> MWILESELFDGKRLWLRPGKTYLFGRTVAEAGQLTISDKTVSRKHLTIHIDNVPEGGGRNLRSRSNVIVEDLESKKGTLVNGVQIRGQKTTLTEDVNEIKLGLCPKTLKIRWHPIVLSFSFTSKELRADPWTNLRDSLEQLDIKYSAEYEPTTTHVVSKKRNTSKGLQALINGRYIVTDSFINAIVQATEIPEGEEGASSALEQDFEANWPNPLDHLPPRGEEPGNHTTETYAPDARRQEVFDGYTFIFYEKKQYDNLFPAISAGKGKALLKEVVPNRTRVDEFVRYVKSVAGEKGLGSFEDGSEGKGVVVVRYTPKGEDSAWYAEFFTKFAQQLDHRPIDQKEFLEAILACDASMLRRPLEAMSQPVSVSASVEPQSSEKVRPAVEDRKEVEQ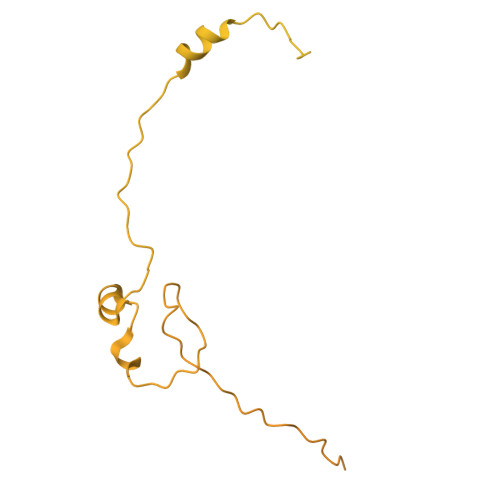SAPKQLQPSAEVPATEESAPAPHRRERRTGRSRFKGFDFDDDDIIIETPQAQSSTQVPALPQVPSASQDSLFVSQREPSLAPSEPMLEEEAPCNTRTTRQTHRKRVLSPLPEHDNSALLDEIAPITAAVKRRRIEAGQDPVPPLPEPEPEREDEDVEMVEESPPRKGKKGAATTAKGKGKKIKQEDEENVLELARRRREEAEAAAAAERQRLAQLGDDDIDYAAIRRLHIIEEIEVRQPEPHGPNRTREQDIADGRWDPRWNGRKNFKRFRRQGETGVRMPVQSVIVPLEEVRTKEYGIGDDYWLEDEEGRVPRRPKETQTQERSTIGSVRDGSGFAAAAASGKGKEKDKENEKEVGRPGSSAAAAKQRSKPAPRRTVLTLDSSDEDEDEPSPHAPGIDTISDSEPEVVSSFPSVIPASEPSRSRAAKAAERANALRSSAHSSQSQTQQHRESQLSTGSSKIQLTLAPGSSSLSFSRSGTAAGRNENGKRPFGSFVSGESTASGRGMSVESGSVRGESASKRQKQGSSGGGSFLATRRKDDGSEEESEDDELKFRFGRRR>MNKWNYGVFFVNFYNKGQQEPSKTMNNALETLRIIDEDTSIYDVINIDDHYLVKKDSEDKKLAPFITLGEKLYVLATSENTVDIAAKYALPLVFKWDDINEERLKLLSFYNASASKYNKNIDLVRHQLMLHVNVNEAETVAKEELKLYIENYVACTQPSNFNGSIDSIIQSNVTGSYKDCLSYVANLAGKFDNTVDFLLCFESMQDQNKKKSVMI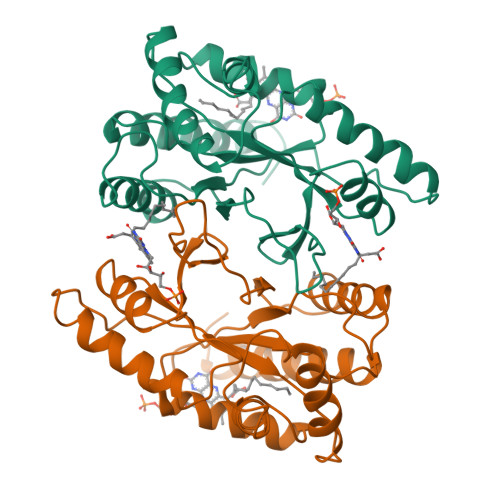DLNNQVIKFRQDNNLI[2x]>[14x]MMGYIPYVIENTDRGERSYDIYSRLLKDRIVLLSGEINDSVASSIVAQLLFLEAEDPEKDIGLYINSPGGVITSGLSIYDTMNFIRPDVSTICIGQAAAMGAFLLSCGAKGKRFS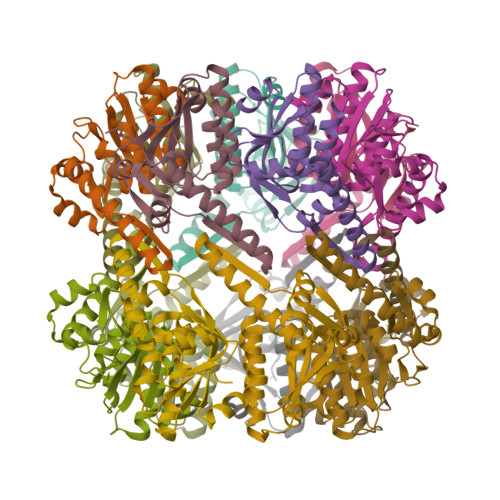LPHSRIMIHQPLGGAQGQASDIEIISNEILRLKGLMNSILAQNSGQSLEQIAKDTDRDFYMSAKEAKEYGLIDKVLQKNVK>MITAQAVLYTQHGEPKDVLFTQSFEIDDDNLAPNEVIVKTLGSPVNPSDINQIQGVYPSKPAKTTGFGTTEPAAPCGNEGLFEVIKVGSNVSSLEAGDWVIPSHVNFGTWRTHALGNDDDFIKLPNPAQSKANGKPNGLTINQGATISVNPLTAYLMLTHYVKLTPGKDWFIQNGGTSAVGKYASQIGKLLNFNSISVIRDRPNLDEVVASLKELGATQVITEDQNNSREFGPTIKEWIKQSGGEAKLALNCVGGKSSTGIARKLNNNGLMLTYGGMSFQPVTIPTSLYIFKNFTSAGFWVTELLKNNKELKTSTLNQIIAWYEEGKLTDAKSIETLYDGTKPLHELYQDGVANSK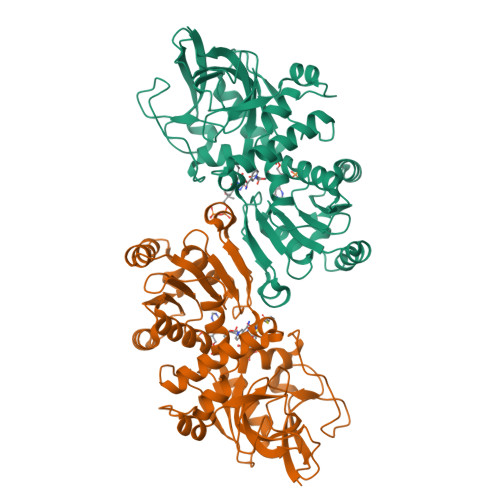DGKQLITY[3x]>SNAQIDGFVRTLRARPEAGGKVPVFVFHPAGGSTVVYEPLLGRLPADTPMYGFERVEGSIEERAQQYVPKLIEMQGDGPYVLVGWSLGGVLAYACAIGLRRLGKDVRFVGLIDAVRAGEEIPQTKEEIRKRWDRYAAFAEKTFNVTIPAIPYEQLEELDNEGQVRFVLDAVSQSGVQIPAGIIEHQRTSYLDNRAIDTAQIQPYDGHVTLYMADRYHDDAIMFEPRYAVRQPDGGWGEYVSDLEVVPIGGEHIQAIDEPIIAKVGEHMSRALGQIEADRTSEVGKQ[2x]

In Mtb, Pks13 performs the final assembly step of mycolic acid synthesis, i.e., the Claisen-type condensation of a C26 α-alkyl branch and C40–60 meromycolate precursors (Portevin et al., 2004). It is comprised of five domains, including two acyl carrier protein domains, a β-ketoacyl-synthase, an acyltransferase, and a C-terminal thioesterase (TE) domain, that together contain all of the activities required for the condensation of two long-chain fatty acids. The overall structure of Pks13-TE consists of a core domain and a lid domain. The Pks13-TE active-site pocket is formed at the interface between the lid and core domains.

Two laboratory-derived mutant strains resistant to TAM1 were found to harbor non-synonymous mutations, i.e., either D1607N or D1644G, both located in the TE domain of Pks13. The crystal structure of the D1607N mutant explained its more subtle effect on binding, through the loss of ion pair interaction between the carboxylate of Asp1607 on helix α6 and the guanidinium of Arg1641 (3 Å) located on the parallel helix, α7. Without this interaction, α7 shifts away from the substrate-binding groove by about 3 Å, moving Asp1644 out of hydrogen-bonding distance from the P4 OH of TAM1.>MSQHNEKNPHQHQSPLHDSSEAKPGMDSLAPEDGSHRPAAEPTPPGAQPTAPGSLKAPDTRNEKLNSLEDVRKGSENYALTTNQGVRIADDQNSLRAGSRGPTLLEDFILREKITHFDHERIPERIVHARGSAAHGYFQPYKSLSDITKADFLSDPNKITPVFVRFSTVQGGAGSADTVRQIRGFATKFYTEEGIFDLVGNNTPIFFIQDAHKFPDFVHAVKPEPHWAIPQGQSAHDTFWDYVSLQPETLHNVMWAMSDRGIPRSYRTMEGFGIHTFRLI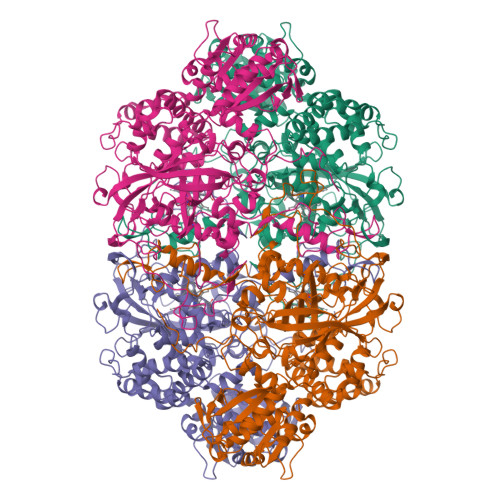NAEGKATFVRFHWKPLAGKASLVWDEAQKLTGRDPDFHRRELWEAIEAGDFPEYELGFQLIPEEDEFKFDFDLLDPTKLIPEELVPVQRVGKMVLNRNPDNFFAENEQAAFHPGHIVPGLDFTNDPLLQGRLFSYTDTQISRLGGPNFHEIPINRPTCPYHNFQRDGMHRMGIDTNPANYEPNSINDNWPRETPPGPKRGGFESYQERVEGNKVRERSPSFGEYYSHPRLFWLSQTPFEQRHIVDGFSFELSKVVRPYIRERVVDQLAHIDLTLAQAVAKNLGIELTDDQLNITPPPDVNGLKKDPSLSLYAIPDGDVKGRVVAILLNDEVRSADLLAILKALKAKGVHAKLLYSRMGEVTADDGTVLPIAATFAGAPSLTVDAVIVPCGNIADIADNGDANYYLMEAYKHLKPIALAGDARKFKATIKIADQGEEGIVEADSADGSFMDELLTLMAAHRVWSRIPKIDKIPA[4x]2-CARBOXYPROPYL-COENZYME A | C25 H42 N7 O18 P3 S 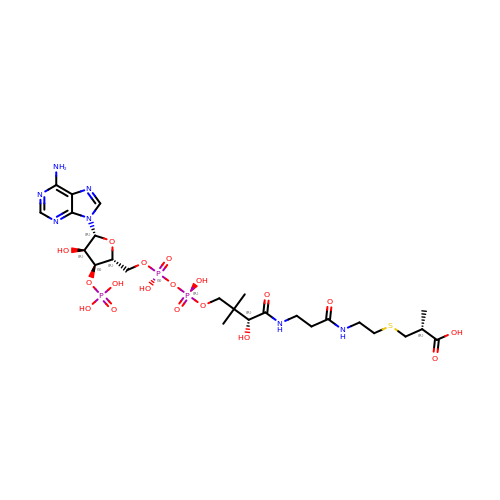| YLEVKEKTOJAHCY-UQCJFRAESA-N>[2x]KDDMKAAEQYQGAASAVDPAHVVRTNG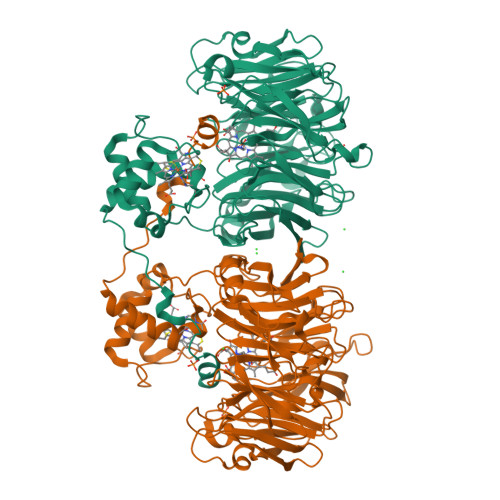APDMSESEFNEAKQIYFQRCAGCHGVLRKGATGKPLTPDITQQRGQQYLEALITYGTPLGMPNWGSSGELSKEQITLMAKYIQHTPPQPPEWGMPEMRESWKVLVKPEDRPKKQLNDLDLPNLFSVTLRDAGQIALVDGDSKKIVKVIDTGYAVHISRMSASGRYLLVIGRDARIDMIDLWAKEPTKVAEIKIGIEARSVESSKFKGYEDRYTIAGAYWPPQFAIMDGETLEPKQIVSTRGMTVDTQTYHPEPRVAAIIASHEHPEFIVNVKETGKVLLVNYKDIDNLTVTSIGAAPFLHDGGWDSSHRYFMTAANNSNKVAVIDSKDRRLSALVDVGKTPHPGRGANFVHPKYGPVWSTSHLGDGSISLIGTDPKNHPQYAWKKVAELQGQGGGSLFIKTHPKSSHLYVDTTFNPDARISQSVAVFDLKNLDAKYQVLPIAEWADLGEGAKRVVQPEYNKRGDEVWFSVWNGKNDSSALVVVDDKTLKLKAVVKDPRLITPTGKFNVYNTQHDVY Serine hydroxymethyltransferase (SHMT or GlyA; EC 2.1.2.1) is a ubiquitous pyridoxal 5’-phosphate (PLP)-dependent enzyme. Its physiologically relevant reaction is the reversible interconversion of serine and tetrahydrofolate (THF) to glycine and 5,10-methylene tetrahydrofolate (MTHF). As MTHF is a major source of cellular one-carbon units, SHMT is a pivotal metabolic enzyme for the biosynthesis of purines and thymidylate. Serine hydroxymethyltransferases, encoded by the glyA genes, are structurally highly conserved, with the active site located at the interface between two monomers.

In order to obtain structural and functional insight into the H. pylori enzyme and address the weak PLP binding observed in purified HpSHMT, we solved the crystal structure of H. pylori SHMT at a resolution of 2.8 Å. HpSHMT crystallized as dimer, like the other known bacterial SHMTs, and no evidence was found for higher oligomeric states in the crystal packing. The HpSHMT structure displays the typical highly conserved overall fold of type I PLP-dependent proteins and is formed by one large and one small domain. Despite sequence conservation of these seven loops, no PLP was present in the HpSHMT structure, providing one of the very few apoprotein structures of an SHMT enzyme. The two active sites of HpSHMT are separated by a distance of 24 Å (calculated between the two PLP α-phosphates), which is considerably longer than the average distance of 18 Å observed in most SHMT structures. This illustrates a modification of the HpSHMT dimer interface, where one subunit is rotated about 17° from the other in comparison to PLP-bound TtSHMT or EcSHMT. Remarkably, loop 1 is completely disordered in the two chains of HpSHMT. Surprisingly, the PLP pocket is found almost pre-organised in one subunit of the HpSHMT structure despite the disorder observed for loops 1, 3 and 7. As a more detailed view of the active site indicates a very strong structural conservation of the residues involved, we propose that the structure of HpSHMT represents an inactive conformation of the enzyme prior to PLP binding.

>MAYFLEQTDSEIFELIFEEYKRQNEHLEMIASENYTFASVMEAMGSVLTNKYAEGYPNKRYYGGCEVVDKIESLAIERAKKLFNCQFANVQAHSGSQANNAVYHALLKPYDKILGMDLSCGGHLTHGAKVSLTGKHYQSFSYGVNLDGYIDYEEALKIAQSVKPEIIVCGFSAYPREIDFKKFREIADEVGALLLGDIAHVAGLVVTGEHAHPFPHCHVVSSTTHKTLRGPRGGIILTNDEEIAAKIDKAIFPGTQGGPLMHVIAAKAVGFKENLKPEFKAYAQLVKSNMQVLAKALKEKNHKLVSGGTSNHLLLMDFLDKPYSGKDADIALGNAGITVNKNTIPGETRSPFVTSGIRIGSAALSARGMGAKEFEIIGNKISDILNDINNVSLQLHVKEELKAMVNQFPVYHQPIFRSHHHHHH[2x]>TYTTRQIGAKNTLEYKVYIEKDGKPVSAFHDIPLYADKENNIFNMVVEIPRWTNAKLEITKEETLNPIIQDTKKGKLRFVRNCFPHHGYIHNYGAFPQTWEDPNVSHPETKAVGDNEPIDVLEIGETIAYTGQVKQVKALGIMALLDEGETDWKVIAIDINDPLAPKLNDIEDVEKYFPGLLRATNEWFRIYKIPDGKPENQFAFSGEAKNKKYALDIIKETHDSWKQLIAGKSSDSKGIDLTNVTLPDTPTYSKAASDAIPPASLKADAPIDKSIDKWF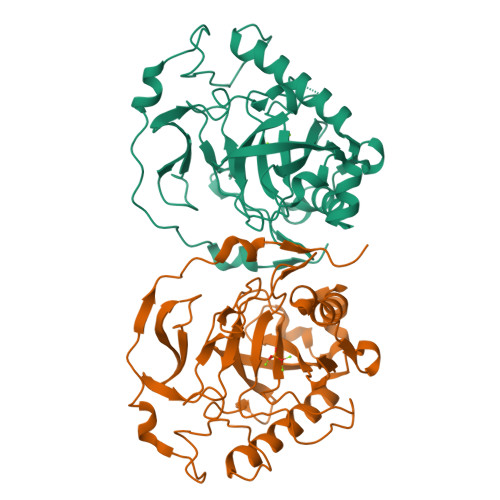FISGSV[2x]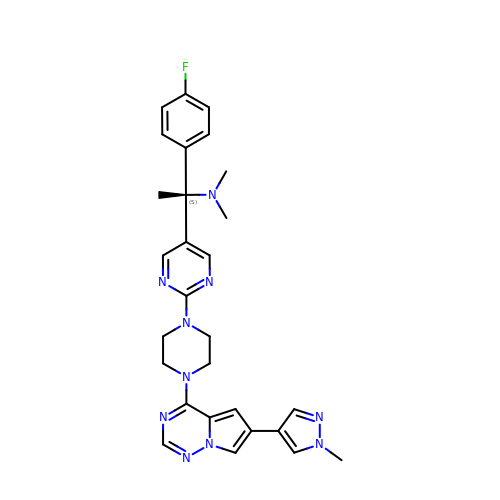(1~{S})-1-(4-fluorophenyl)-~{N},~{N}-dimethyl-1-[2-[4-[6-(1-methylpyrazol-4-yl)pyrrolo[2,1-f][1,2,4]triazin-4-yl]piperazin-1-yl]pyrimidin-5-yl]ethanamine | C28 H31 F N10 | UDARLCIFKQITPT-NDEPHWFRSA-N>YEQDKTYKITVLHTNDHHGHFWRNEYGEYGLAAQKTLVDGIRKEVAAEGGSVLLLSGGDINTGVCESDLQDAEPDFRGMNLVGYDAMAIGNHEFDNPLTVLRQQEKWAKFPLLSANIYQKSTGERLFKPWALFKRQDLKIAVIGLTTDDTAKIGNPEYFTDIEFRKPADEAKLVIQELQQTEKPDIIIAATHMGHYDNGEHGSNAPGDVEMARALPAGSLAMIVGGHSQDPVCMAAENKKQVDYVPGTPCKPDQQNGIWIVQAHEWGKYVGRADFEFRNGEMKMVNYQLIPVNLKKKVTWEDGKSERVLY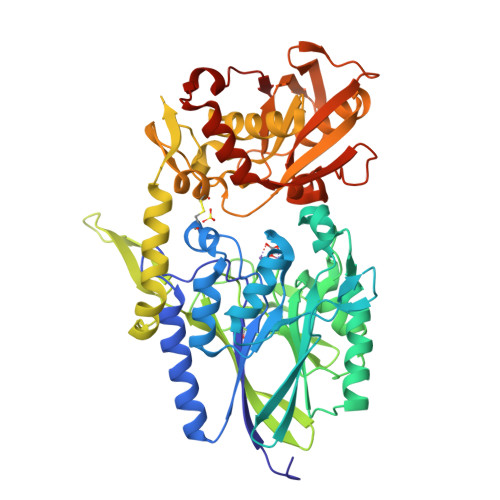TPEIAENQQMISLLSPFQNKGKAQLEVKIGETNGRLEGDRDKVRFVQTNMGRLILAAQMDRTGADFAVMSGGGIRDSIEAGDISYKNVCKVQPFGNVVVYADMTGKEVIDYLTAVAQMKPDSGAYPQFANVSFVAKDGKLNDLKIKGEPVDPAKTYRMATLNFNATGGDGYPRLDNKPGYVNTGFIDAEVLKAYIQKSSPLDVSVYEPKGEVSWQEHHHHHH[2x]> MKSVITTVVSAADAAGRFPSNSDLESIQGNIQRSAARLEAAEKLAGNHEA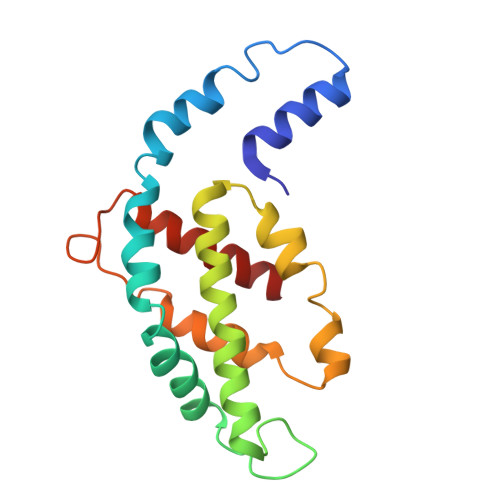VVKEAGDACFAKYAYLKNPGEAGENQEKINKCYRDVDHYMRLVNYCLVVGGTGPLDEWGIAGAREVYRTLNLPTSAYVASIAYTRDRLCVPRDMSAQAGVEFSAYLDYLINALS>MKGQTQRSVLLCKVVGACGVGKSAFLQAFLGRGLGHQDTREQPPGYAIDTVQVNGQEKYLILCEVGTDGLLATSLDATCDVACLMFDGSDPKSFAHCASVYKHHYMDGQTPCLFVSSKADLPEGVAVSGPSP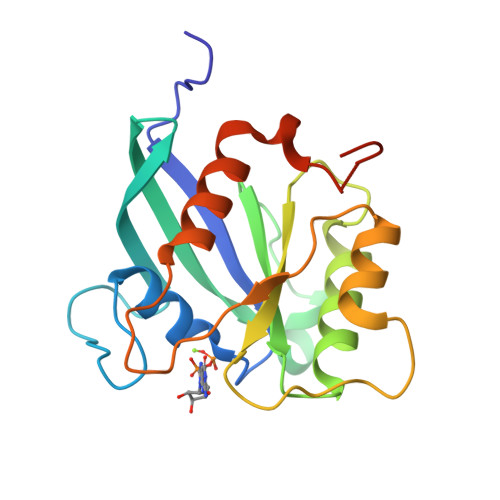AEFCRKHRLPAPVPFSCAGPAEPSTTIFTQLATMAAFPHLVHAELHPSSLEHHHHHH[3x]>ALSAKLTLDKVDLKGKRVIMRVDFNVPMKNNQITNNQRIKAAIPSIKHCLDNGAKSVVLMSHLGRPDGIPMPDKYSLEPVADELKSLLNKDVIFLKDCVGPEVEQACANPDNGSIILLENLRFHVEEEGKGKDSSGKKISADPAKVEAFRASLSKLGDVYVNDAFGTAHRAHSSMVGVNLPQKASGFLMKKELDYFSKALEKPERPFLAILGGAKVKDKIQLIKNMLDKVNFMIIGGGMAYTFLKELKNMQIGASLFDEEGATIVKEIMEKAEKNGVKIVFPVDFVTGDKFDENAKVGQATIESGIPSGWMGLDCGPESIKINAQIVAQAKLIVWNGPIGVFEWDAFAKGTKALMDEVVKATSNGCVTIIGGGDTATCCAKWGTEDKVSHVSTGGGASL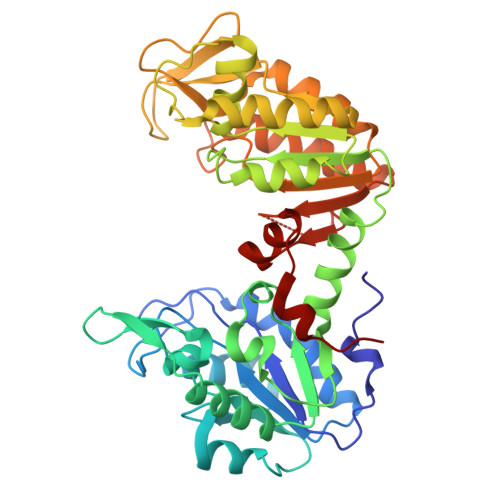ELLEGKILPGVEALSNM[2x]3-(beta-D-glucopyranosyl)-6-pentylfuro[2,3-d]pyrimidin-2(3H)-one | C17 H24 N2 O7 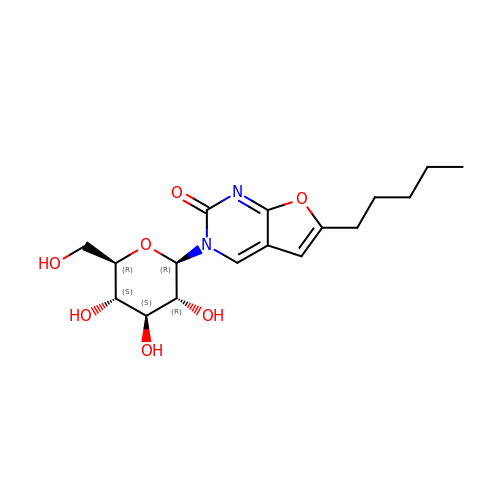| OPBPIQMYHFDOAO-XYFZXANASA-N> MEAVLNELVS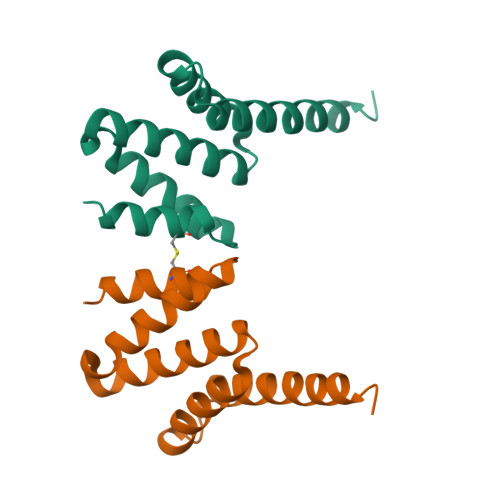VEDLLKFEKKFQSEKAAGSVSKSEQFEYAWCLVRSKYNDDIRKGIVLLEELLPKGSKEEQRDYVFYLAVGNYRLKEYEKALKYVRGLLQTEPQNNQAKELERLIDKAMKKDGLLEVLFQ> GPAMSVPAIAPRRKRLADGLSVTQKVFVRSRNGGATKIVREHYLRSDIPCLSRSCTKCPQIVVPDAQNELPKFILSDSPLELSAPIGKHYVVLDTNVVLQAIDLLENPNCFFDVIVPQIVLDEVRNKSYPVYTRLRTLCRDSDDHKRFIVFHNEFSEHTFVERLPNETINDRNNRAIRKTCQWYSEHLKPYDINVVLVTNDRLNREAATKEVESNIITKSLVQYIELLPNADDIRDSIPQMDSFDKDLERDTFSDFTFPEYYSTARVMGGLKNGVLYQGNIQISEYNFLEGSVSLPRFSKPVLIVGQKNLNRAFNGDQVIVELLPQSEWKAPSSIVLDSEHFDVNDNPDIEAGDDDDNNESSSNTTVISDKQRRLLAKDAMIAQRSKKIQPTAKVVYIQRRSWRQYVGQLAPSSVDPQSSSTQNVFVILMDKCLPKVRIRTRRAAELLDKRIVISIDSWPTTHKYPLGHFVRDLGTIESAQAETEALLLEHDVEYRPFSKKVLECLPAEGHDWKAPTKLDDPEAVSKDPLLTKRKDLRDKLICSIDPPGCVDINDALHAKKLPNGNWEVGVHIADVTHFVKPGTALDAEGAARGTSVYLVDKRIDMLPMLLGTDLCSLKPYVDRFAFSVIWELDDSANIVNVNFMKSVIRSREAFSYEQAQLRIDDKTQNDELTMGMRALLKLSVKLKQKRLEAGALNLASPEVKVHMDSETSDPNEVE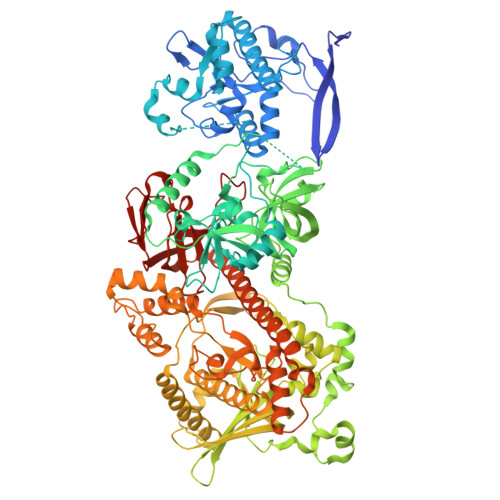IKKLLATNSLVEEFMLLANISVARKIYDAFPQTAMLRRHAAPPSTNFEILNEMLNTRKNMSISLESSKALADSLDRCVDPEDPYFNTLVRIMSTRCMMAAQYFYSGAYSYPDFRHYGLAVDIYTHFTSPIRRYCDVVAHRQLAGAIGYEPLSLTHRDKNKMDMICRNINRKHRNAQFAGRASIEYYVGQVMRNNESTETGYVIKVFNNGIVVLVPKFGVEGLIRLDNLTEDPNSAAFDEVEYKLTFVPTNSDKPRDVYVFDKVEVQVRSVMDPITSKRKAELLLK>[2x]SHHHHHHGESLFKGPRDYNPISSTICHLTNESDGHTTSLYGIGFGPFIITNKHLFRRNNGTLLVQSLHGVFKVKNTTTLQQHLI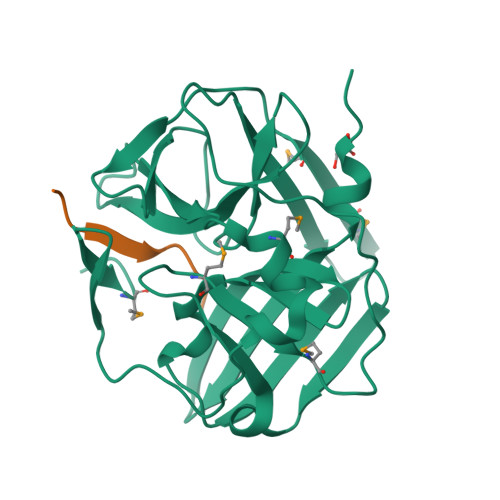DGRDMIIIRMPKDFPPFPQKLKFREPQREERICLVTTNFQTKSMSSMVSDTSCTFPSSDGIFWKHWIQTKDGQAGSPLVSTRDGFIVGIHSASNFTNTNNYFTSVPKNFMELLTNQEAQQWVSGWRLNADSVLWGGHKVFMSKPEEPFQPVKEATQLMN;>TENLYFQSGT[2x]N-[(1S,2R)-1-BENZYL-3-(CYCLOPROPYLAMINO)-2-HYDROXYPROPYL]-5-[METHYL(METHYLSULFONYL)AMINO]-N'-[(1R)-1-PHENYLETHYL]ISOPHTHALAMIDE 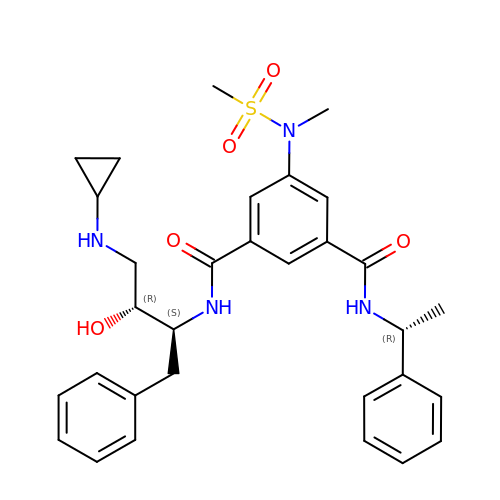| C31 H38 N4 O5 S | VPNIQGRFZCTBEZ-SPTGULJVSA-N>MTKSLFRQSFLTDTLDVHIDVAPAEQVLSNGVQLKLYQRGVLEVIPENPTQETKNIIISCGIHGDETAPMELVDSIIK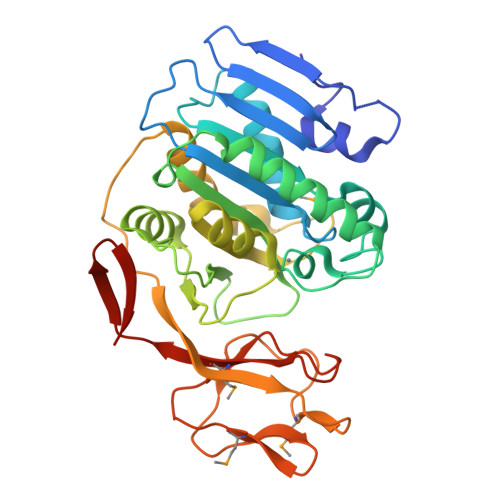DIESGFQKVDARCLFIIAHPESTLAHTRFLEENLNRLFDEKEHEPTKELAIADTLKLLVRDFYQDTEPKTRWHLDLHCAIRGSKHYTFAVSPKTRHPVRSKALVDFLDSAHIEAVLLSNSPSSTFSWYSAENYSAQALTMELGRVARIGENALDRLTAFDLALRNLIAEAQPEHLSKPCIKYRVSRTIVRLHDDFDFMFDDNVENFTSFVHGEVFGHDGDKPLMAKNDNEAIVFPNRHVAIGQRAALMVCEVKTRFEEGELVYDLEHHHHHH[2x]> MAMSNGNNDFVVLSNSSIATSAANPSPLTPCDGDHAAQQLTPKEATRTKVSPNGCLQLNGTVKSSFLPLDNQRMPQMLPQCCHPCPYHHPLTSHSSHQECHPEAGPAAPSALASCCMQPHSEYSASLCPNHSPVYQTTCCLQPSPSFCLHHPWPDHFQHQPVQQHIANIRPSRPFKLPKSYAALIADWPVVVLGMCTMFIVVCALVGVLVPELPDFSDPLLGFEPRGTAIGQRLVTWNNMVKNTGYKATLANYPFKYADEQASSLEVLFQ;> GPGSEVDWNFHKDSFFCDVPSDRYSRVVFTSSGGETLWNLPAIKSMCNVDNSRIRSHPQFGDLCQRTTAASCCPSWTLGNYIAILNNRSSCQKIVERDVSHTLKLLRTCAKHYQNGTLGPDCWDMAARRKDQLKCTNVPRKCTKYNAVYQILHYLVDKDFMTPKTADYATPALKYSMLFSPTEKGESMMNIYLDNFENWNSSDGVTTITGIEFGIKHSLFQDYLLMDTVYPAIAIVIVLLVMCVYTKSMFITLMTMFAIISSLIVSYFLYRVVFHFEFFPFMNLTALIILVGIGANNAFVLCDVWNYTKFDK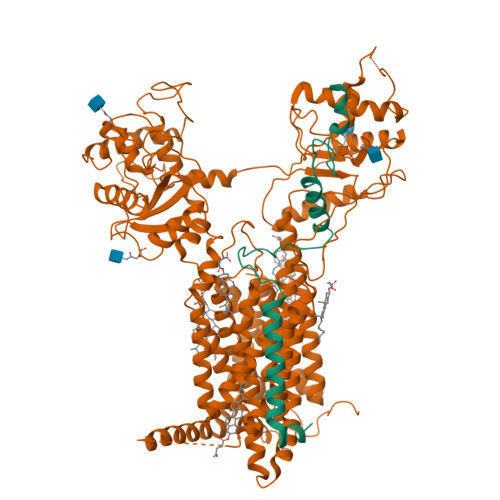PHAETSETVSITLQHAALSMFVTSFTTAAAFYANYVSNITAIRCFGVYAGTAILVNYVLMVTWLPAVVVLHERYLLNIFTCFKKPQQQIYDNKSCWTVACQKCHKVLFAISEASRIFFEKVLPCIVIKFRYLWLFWFLALTVGGAYIVCINPKMKLPSLELSEFQVFRSSHPFERYDAEYKKLFMFERVHHGEELHMPITVIWGVSPEDNGNPLNPKSKGKLTLDSSFNIASPASQAWILHFCQKLRNQTFFYQTDEQDFTSCFIETFKQWMENQDCDEPALYPCCSHWSFPYKQEIFELCIKRAIMELERSTGYHLDSKTPGPRFDINDTIRAVVLEFQSTYLFTLAYEKMHQFYKEVDSWISSELSSAPEGLSNGWFVSNLEFYDLQDSLSDGTLIAMGLSVAVAFSVMLLTTWNIIISLYAIISIAGTIFVTVGSLVLLGWELNVLESVTISVAVGLSVNFAVHYGVAYRLAPDPDREGKVIFSLSRVGSAMAMAALTTFVAGAMMMPSTVLAYTQLGTFMMLIMCISWAFATFFFQCMCRCLGPQGTCGQIPLPKKLQCSAFSHALSTSPSDKGQSKTHTINAYHLDPRGPKSELEHEFYELEPLASHSCTAPEKTTYEETHICSEFFNSQAKNLGMPVHAAYNSELSKSTESDAGSALLQPPLEQHTVCHFFSLNQRCSCPDAYKHLNYGPHSCQQMGDCLCHQCSPTTSSFVQIQNGVAPLKATHQAVEGFVHPITHIHHCPCLQGRVKPAGMQNSLPRNFFLHPVQHIQAQEKIGKTNVHSLQRSIEEHLPKMAEPSSFVCRSTGSLLKTCCDPENKQRELCKNRDVSNLESSGGTENKAGGKVELSLSQTDASVNSEHFNQNEPKVLFNHLMGEAGCRSCPNNSQSCGRIVRVKCNSVDCQMPNMEANVPAVLTHSELSGESLLIKTL> MAEASSANLGSGCEEKR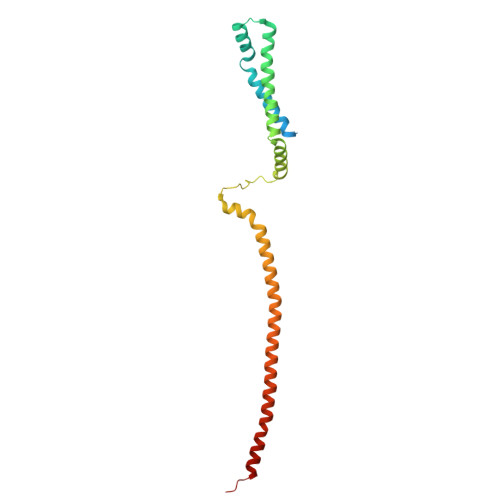HEGSSSESVPPGTTISRVKLLDTMVDTFLQKLVAAGSYQRFTDCYKCFYQLQPAMTQQIYDKFIAQLQTSIREEISDIKEEGNLEAVLNALDKIVEEGKVRKEPAWRPSGIPEKDLHSVMAPYFLQQRDTLRRHVQKQEAENQQLADAVLAGRRQVEELQLQVQAQQQAWQALHREQRELVAVLREPE guanosine 5'-(tetrahydrogen triphosphate) 3'-(trihydrogen diphosphate) 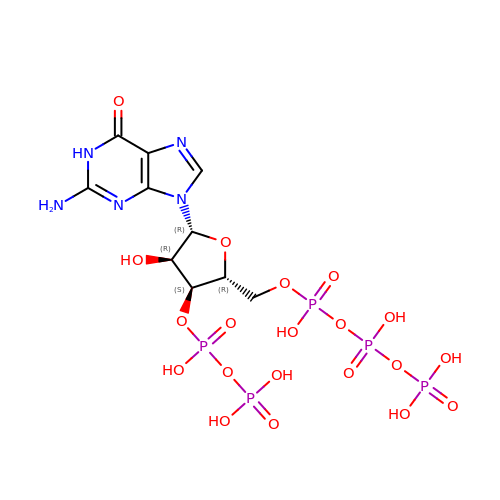| C10 H18 N5 O20 P5 | KCPMACXZAITQAX-UUOKFMHZSA-N> HHHHHHTGQENKQENKRSFFDFLKYKTIKEDDLNDVIEELRFQLLDSDVSYEVTEKILEDLKNNLIGKKVSRREEVEEIVINTLKKSITEILTKNQKTDLIEKIRSSGKKPFVIIFFGVNGVGKTTTIAKVVNMLKKNNLSTIIAASDTFRAAAQEQLAYHASKLEVQLIRGKYGADPASVAFDAISFAKSRNIDVVLIDTAGRMHIDSDLVEELKRVLRIAKPDFRILILDSLAGSDALEQARHFENNVGYDAVILTKVDADAKGGIALSLAYE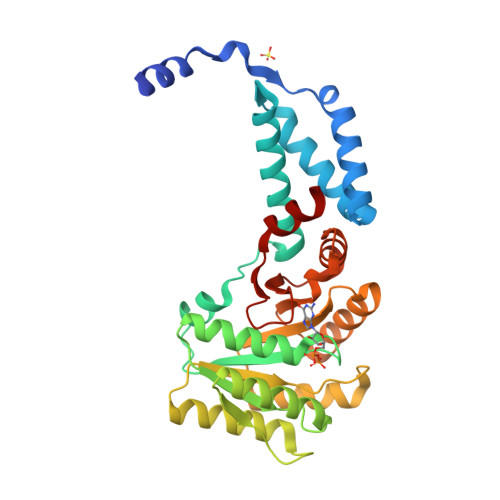LKKPVVYMGVGQNYDDLIPFSPDWFVERIFS>[6x]MRGSHHHHHHGSMDNAFSPSDLKT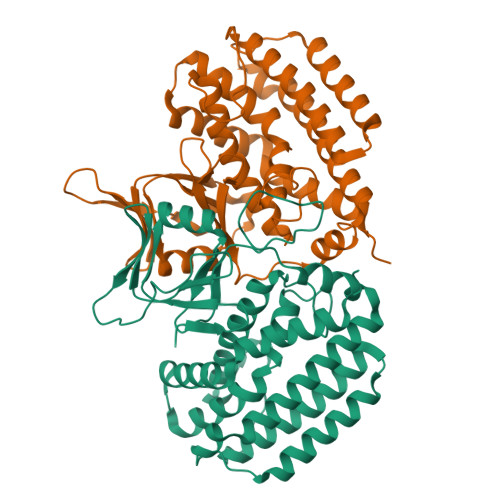ILHSKRANVYYLQHCRILVNGGRVEYVTEEGNQSLYWNIPIANTSVVMLGTGTSVTQAAMREFARAGVMIGFCGGGGTPLFAANEAEVAVSWLSPQSEYRPTEYLQDWVSFWFDDEKRLAAAIAFQQVRITQIRQHWLGSRLSRESRFTFKSEHLQALLDRYQKGLTDCRTSNDVLVQEAMMTKALYRLAANAVSYGDFTRAKRGGGTDLANRFLDHGNYLAYGLAAVSTWVLGLPHGLAVLHGKTRRGGLVFDVADLIKDALVLPQAFIAAMEGEDEQEFRQRCLTAFQQSEALDVMIGSLQDVASKLSQVVR> MEPHDTLSPAQVDEYRKNGFLVQEHVFDEEEIELLRAEAAQEFASGGERVTVEQNTGIVRGVHGCHLYSEVFGRLVRSPRLLPIARQLLRDDVYVHQFKINAKRAFKGEVWEWHQDYTFW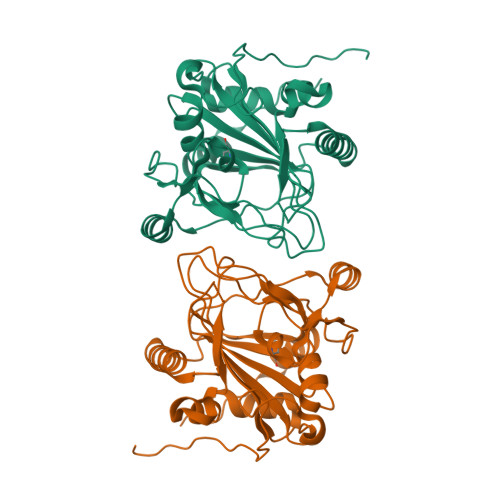HHEDGMPAPRALSAAIFLDEVTEFNGPLTFVPGGHGSGMIDADVKGEGWANTLTASLKYSLDVETMRGLIERNGMVAPKGPRGSVLWFDANIPHSSVPNISPFDRGLVLITYNSVENKTDVTRGTRPEWLAARDFTPLTALQATSF> MPSEQRGQHRSGYGLGLSTRTQVTGYQFLARRTAMALTRWRVRMEVEPGRRQVLAVVASVSAAGVICLGALLWSFISPSGQMGESPIIADRDSGALYVRVGDTLYPALNLASARLIAGRAENPHKVRSSQIAEQPHGPMVGIPGAPSDISPTSPASSSWLVCDAVTAAQGVGAPASVTVTVIDGTPDLSGRRHVLSGSDAVVLRYGNDTWVIRQGRRSRIDAANRAVLLPLGLTPEQVKQASPMSRALYDALPVGPELAVPKVPDAGKPANFPGAPAPVGAVLVTPQISGPQQYSVVLPDGVQTISPIVAQILQNAGTPAGSMPVVVAPATLARMPVVHGLDLSAYPDSPLNVVNMKENPATCWWWEKTAGEERARTQVVSGPTVPIATSDTNKVVSLVKADNTGREADRVYYGPNYANFVVVTGNDPAASTAESLWLLSKSGVRFGVDNSREARTALGLTSTPSPAPWVALRLLAPGPMLSRADALVRHDTLPTDTNPAELAVPK;> MKQGFARPTPERAPVVKPENIVLPTPLSVPPPEGKPWWLVVVGVLVVGLLVGMVGMTVASGSRLFLGAGAIFPIFMIGGVAMMMFGGRFGGQQQMSRPKLDAMRAQFMLMLDMLRETAQESADSMDANYRWFHPAPTTLAAAVGSSRMWERQPDGKDLNFGVVRVGVGMTRPEVTWGEPQNMPTDIELEPVTGKALQEFGRYQSVVYNLPKMVSLLVEPWYSLVGEREQVLGLTRAIICQLAFSHGPDHVQMIVVTSDPDRWDWVKWIPHFGDPRRRDAAGNARMVYTSVREFATEQAELFAGRGSFTPRHASSSAETPTPHHVIISDIEDPQWEYVISSEGVDGVTFFDLTGSPLWTGAPQRVLRFTDSAGVIETLPRDRDTWMVIDDNAWFFALA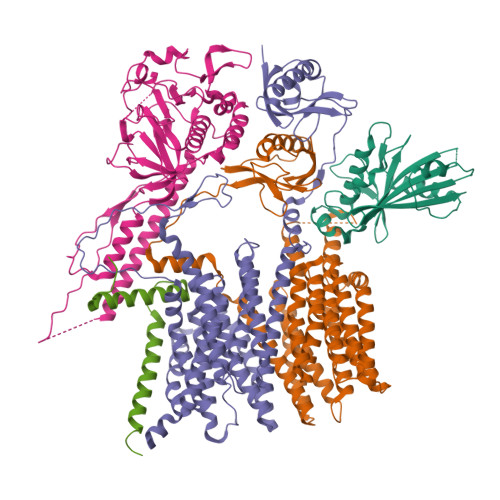DQMSEADAEQFAHQMAHWRLAEAYEEIGQRVVQLGARDILSYYGIDDAGEIDFNTLWSGSGRRDLLSRSRLRIPFGNRADNGELLFLDMKSLDEGGDGPHGVMSGTTGSGKSSLVRTVIASLMLAHPPEELQFVLADLKGGSAVKPFDGVPHVSRIITDLEDDQALMERFLEAMWGEIARRKEICFSAGVDGAKEYNELRARMKARGEDMPPLPMLVVVIDEFYEWFRIMPTAVDVLDSIGRQGRAYWVHLMMASQTIESRAEKLMENMGYRLVLKAQTAGAAQAAGVPNAVNLPSQAGLGYFRKSGDEIIRFQAEYLWRDYRRGSSYDGEEQAPLTHSVDYIRPQLFTTAFAPLEVSVSGPDGQSALPQVVDGEAVNGHRGGDDVDEEEEALRTPKVGTVIIDQLRQIDFEPYRLWHPPLDVPVPIDELVNRFLGRPWQQDYGTAKNLVFPIGIIDRPYKHDQPPWTVDTSGAGANVLILGAGGAGKTTALQTLICAAALTHTPEQVQFYCLAYSGTALTTVANLPHVGGVSGPTDPYGVRRTVAEVLGLVRDRKRSFLEYDVPSMEVFRRRKFGGEPGGVPDDGFGDVYLVIDNYRALAEENEVLIEQVNQIINQGPSFGVHVVATADRESELRPPVRSGFGSRVELRLAAVEDAKLVRSRFAKDVPPKPGRGMVAVNYVRLDSDPQAGLHTLVARPALGSTPDAVFESDSVAAAVRQVAAGEARPVRRLPARFGLDQLRQVAAADRRQGVGAGGIAWAISELDLQPVYLNFADNAHLMVTGRRECGRTTTLATIMSEIGRIYAPGASTAPPTSRPSAQVWLVDPRRQLLTVLGSDYVEKFAYNLDGVAAMMDDLAAALARREPPPGLSAEELLSRSWWSGPEIFLIIDDIQQLPPGFDSPLHKAAPWVTRAADVGLHVFVTRTFGGWSSAGSDPILRALHQANAPLLVMDADPDEGFIRGKMKGGPLPRGRGLLMAEDTGVFVQVAATDLRR;>MTAIVEAPQPGAEAIASPQAAVVAIMAADVQIAVVLDAHAPISVMIDPLLKVVNTRLRELGVAPLEAKGRGRWMLCLVDGTPLRPNLSLTEQEVYDGDRLWLKFLEDTEHRSEVIEHISTAVATNLSKRFAPIDPVVAVQVGATMVAVGVLLGSALLGWWRWQHESWLPAPFAAVIAVLVLTVATMILARSKTVPDRRVGDILLLSGLVPLAVAIAATAPGPVGAPHAVLGFGVFGVAAMLVMRFTGRRLGVYTALVTLCAAATAAGLARMVLLTSAVTLLTCVLLACVLMYHGAPALSRWLSGIRLPVFPSATSRWVFEARPDLPTTVVVSGGGQPTLEGPASVRDVLLRAERARSFLTGLLVGLGVLTVVCLAGLCDPHAGRRWLPLLLAAFTFGFLILRGRSYVDRWQAITLAATAVLIIAAVAVRYVLVSGSPAVLSAGVAVLVLLPAAGLTAAAVVPNTIYSPLFRKIVEWIEYLCLMPIFPLALWLMNVYEAIRYR[2x];> MRAQRRFGLDLSWPRLTGVFLIDVAVLALVSHLPDAWQANHIAWWTGVGVAVLVTIVAVVTYRRTPLACALVARVLDRFVDPEMTLTEGCTPALDHQRRFGHDVVGIREYQGQLVAVVTVEGHEEAPSGRHRNRDAAPAWLPVEAVAARLRQFDVRLDAIDIVSVGTRRTSGRDDVSDVGVDDTGPVDARQPLDEHHTWLVLRMDPQRNVAAVAARDSVAATLAAATERLAHDLNGRRWTARPLTSSEIDDMDATVLAGLQPAHVRPRRRRLKYKQPEGYKEFVTSFWVSPRDITSETLERLWLPDTEATAVTVRLRPRHGGVEVSAWVRYHSSRRLRRSVWGGLNRLTGRQLDAVCASMPVPTRRPRLVVPARELHDGEELAVLVGQAPAPSPSPAAAR>MFSNKTRQDSIQKMQQEELDLLIIGGGITGAGVAVQAAASGIKTGLIEMQDFAEGTSSRSTKLVHGGIRYLKTFDVEVVADTVGERAVVQGIAPHIPKPDPMLLPIYEDEGATTFNMFSVKVAMDLYDKLANVTGTKYENYTLTPEEVLEREPFLKKEGLKGAGVYLDFRNNDARLVIDNIKKAAEDGAYLVSKMKAVGFLYEGDQIVGVKARDLLTDEVIEIKAKLVINTSGPWVDKVRNLNFTRPVSPKMRPTKGIHLVVDAKKLPVPQPTYFDTGKQDG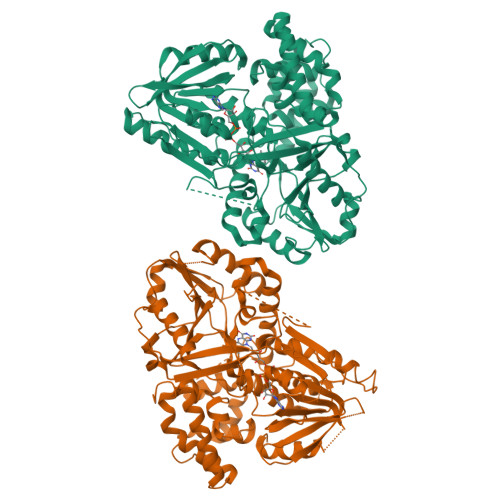RMVFAIPRENKTYFGTTDTDYQGDFTDPKVTQEDVDYLLDVINHRYPEANITLADIEASWAGLRPLLIGNSGSDYNGGDNGSISDKSFNKVVDTVSEYKENKVSRAEVEDVLNHLENSRDEKAPSTISRGSSLEREPDGLLTLSGGKITDYRKMAEGALRLIRQLLKEEYGIETKEIDSKKYQISGGNFDPTKLEETVTELAKEGVAAGLEEEDATYIADFYGTNARRIFELAKEMAPYPGLSLAESARLRYGLEEEMVLAPGDYLIRRTNHLLFERDQLDEIKQPVIDAIAEYFGWTEEEKAQQTKRLEALIAESDLRELKGEK[2x]> TVAYIAIGSNLASPLEQVNAALKALGDIPESHILTVSSFYRTP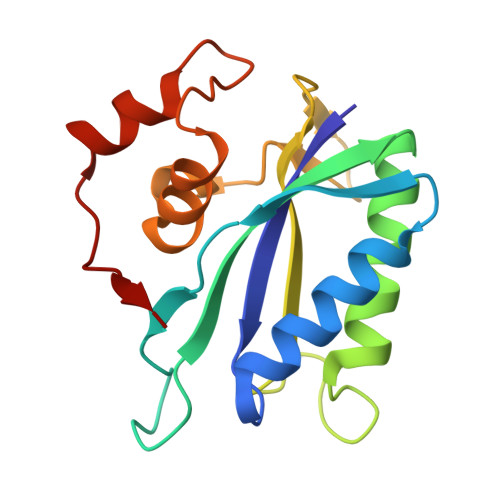PLGPQDQPDYLNAAVALETSLAPEELLNHTQRIELQQGRVRKAERWGPRTLDLDIMLFGNEVINTERLTVPAYDMKNRGFMLWPLFEIAPELVFPDGEMLRQILHTRAFDKLNKW> AERPTLPIPDLLTTDARNRIQLTIGAGQSTFGGKTATTWGYNGNLLGPAVKLQRGKAVTVDIYNQLTEETTLHWHGLEVPGEVDGGPQGIIPPGGKRSVTLNVDQPAATCWFHPHQHGKTGRQVAMGLAGLVVIEDDEILKLMLPKQWGIDDVPVIVQDKKFSADGQIDYQLDVMTAAVGWFGDTLLTNGAIYPQHAAPRGWLRLRLLNGCNARSLNFATSDNRPLYVIASDGGLLPEPVKVSELPVLMGERFEVLVEVNDNKPFDLVTLPVSQMGMAIAPFDKPHPVMRIQPIAISASGALPDTLSSLPALPSLEGLTVRKLQLSMDPMLDMMGMQMLMEKYGDQAMAGMDHSQMMGHMGHGNMNHMNHGGKFDFHHANKINGQAFDMNKPMFAAAKGQYERWVISGVGDMLLHPFH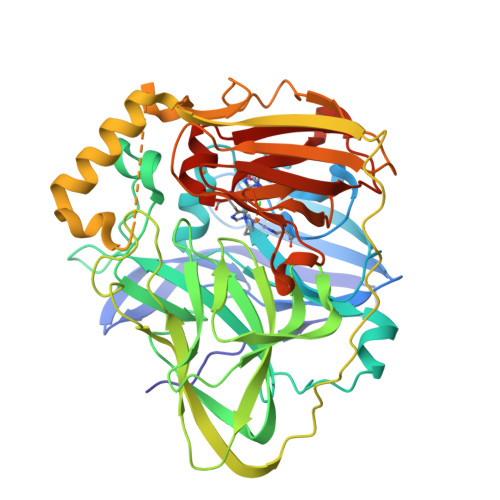IHGTQFRILSENGKPPAAHRAGWKDTVKVEGNVSEVLVKFNHDAPKEHAYMAHCHLLEHEDTGMMLGFTVSAWSHPNFEK> MQDAITAVINASDVQGKYLDSSALDRLKSYFQSGELRVR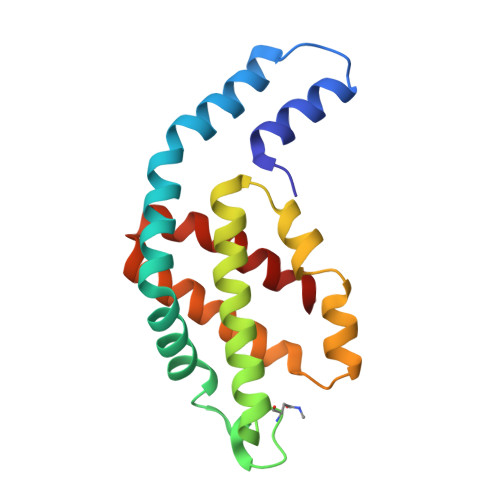AAATISANSALIVKEAVAKSLLYSDITRPGGNMYTTRRYAACIRDLEYYLRYATYAMLAGDTSILDERVLNGLKETYNSLGVPIGATVQAIQAIKEVTASLVGPDAGREMGVYLDYISSGLS>[2x]MVIATIQAEDHSQQSGTQQETTTDTGGGKNVGYIDAGDWLSYAGTPVNIPSSGSYLIEYRVASQ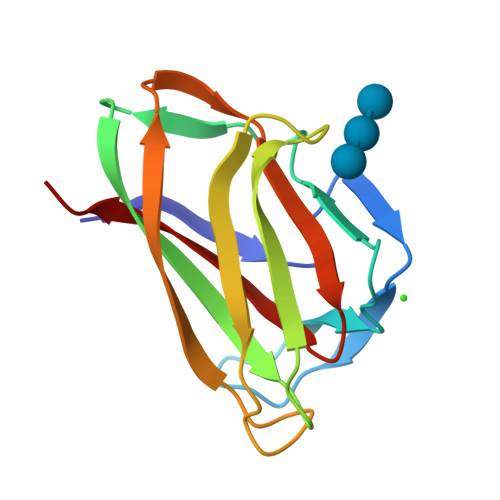NGGGSLTFEEAGGAPVHGTIAIPATGGWQTWTTIQHTVNLSAGSHQFGIKANAGGWNLNWIRINKTH N-{(1S)-5-[(2-fluoro-6-hydroxybenzene-1-carbonyl)amino]-1-[5-(naphthalen-2-yl)-1H-imidazol-2-yl]pentyl}-1,3-thiazole-5-carboxamide | C29 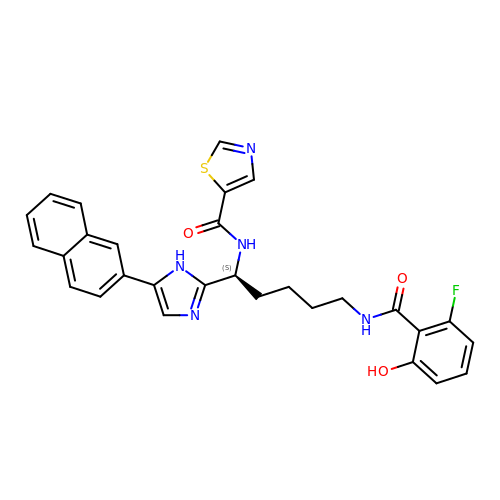H26 F N5 O3 S | BBLOAIWXSMVTHJ-QFIPXVFZSA-N> MLEANVYDNFNPNYYNISDFSMPNGKKEKRGLPIPKARCQVINYELWETGYLYTSSATLTVSVEVGDIVQILFPEVVPIEEALGKKKKLNLDMVYLVTDVDESNKATLKNYFWAMIESLDVPNAITKT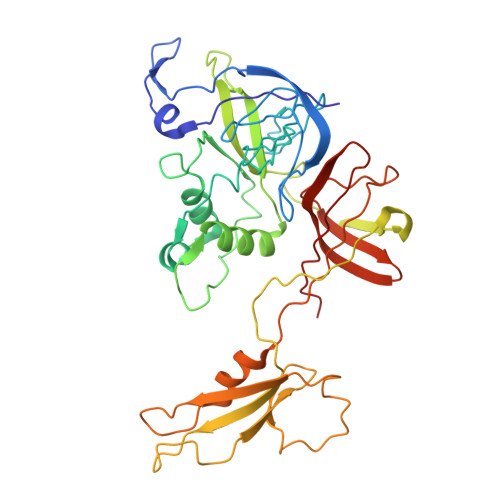TNFAIIDYLIDPNKNNLMSYGYFFNSSIFAGKATINRKAETSSAHDVAKRIFSKVQFQPTTTIQHAPSETDPRNLLFINFASRNWNRKRITTRVDIKQSVTMDTETIVDRSAYNFAVVFVKNKATDDYTDPPKMYIAKNNGDVIDYSTYHGDGTDLPDVRTAKTLFYDRDDHGNPPELSTIKVEISPSTIVTRLIFNQNELLPLYVNDLVDIWYEGKLYSGYIADRVKTEFNDRLIFVESGDKPNVI> GRGDS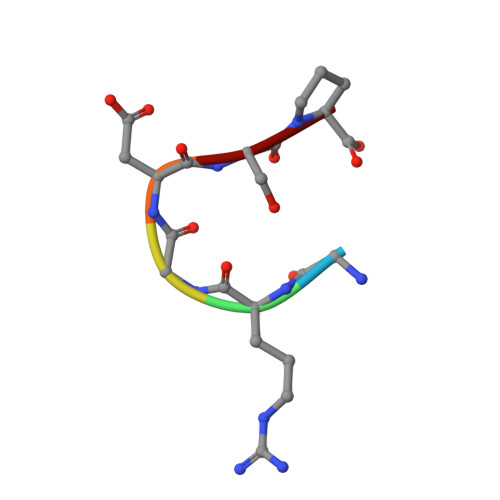P>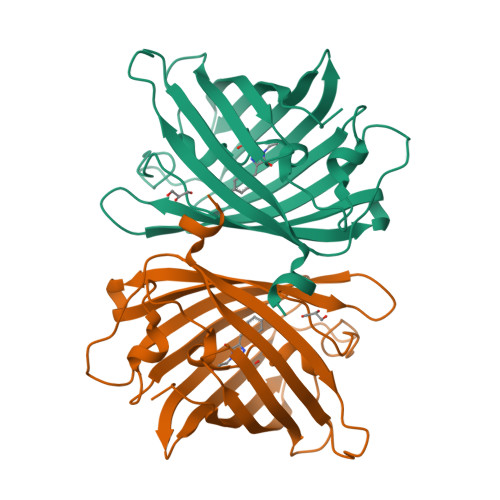[4x]MSYGALLFREKIPYVVEMEGDVEGMKFSVRGKGHGDANTGKIEASFICTTGELPVPWSSILTTVTYGAQCFAKYPNDIKDYPKSAMPEGYVQERTITFENDGVYKTRAEVTYEKGSVYNRVTLNGSGFKKGGNILGKKLEFNYNPHCIYVLPDVQNNGIKCYINIVHDVIGGGQIIAAHQQLNTPLGGGPVDIPHYHHIQAHTILSKDPKETRDHMNVVEVFRAIDCKTAYA>MTKYRLSEGPRAFTYQVDGEKKSVLLRQVIAVTDFNDVKAGTSGGWVDADNVLSQQGDCWIYDENAMAFAGTEITGNARITQPCTLYNNVRIGDNVWIDRADISDGARISDNVTIQSSSVREECAIYGDARVLNQSEILAIQGLTHEHAQILQIYDRATVNHSRIVHQVQLYGNATITHAFIEHRAEVFDFALIEGDKDNNVWICDCAKVYGHARVIAGTEEDAIPTLRYSSQVAEHALIEGNCVLKHHVLVGGHAEVRGGPILLDDRVLIEGHACIQGEILIERQVEISGRAAVIAFDDNTIHLRGPKVINGEDRITRTPLVGSLLEHHHHHH[2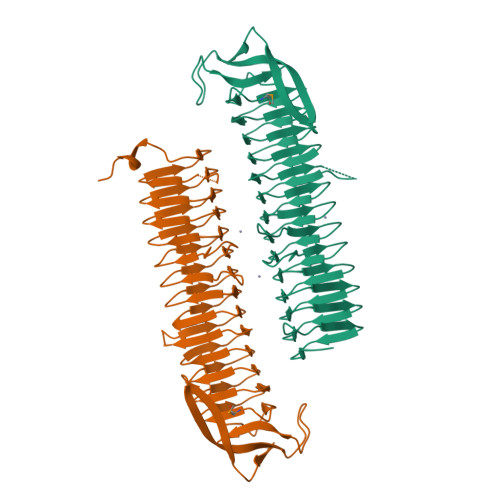x]> MASMTGGQQMGRGSMPEIVDTCSLASPASVCRTKHLHLRCSVDFTRRTLTGTAALTVQSQEDNLRSLVLDTKDLTIEKVVINGQEVKYALGERQSYKGSPMEISLPIALSKNQEIVIEISFETSPKSSALQWLTPEQTSGKEHPYLFSQCQAIHCRAILPCQDTPSVKLT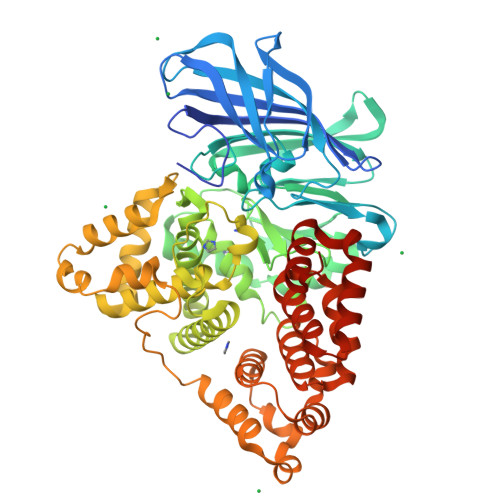YTAEVSVPKELVALMSAIRDGETPDPEDPSRKIYKFIQKVPIPCYLIALVVGALESRQIGPRTLVWSEKEQVEKSAYEFSETESMLKIAEDLGGPYVWGQYDLLVLPPSFPYGGMENPCLTFVTPTLLAGDKSLSNVIAHEISHSWTGNLVTNKTWDHFWLNEGHTVYLERHICGRLFGEKFRHFNALGGWGELQNSVKTFGETHPFTKLVVDLTDIDPDVAYSSVPYEKGFALLFYLEQLLGGPEIFLGFLKAYVEKFSYKSITTDDWKDFLYSYFKDKVDVLNQVDWNAWLYSPGLPPIKPNYDMTLTNACIALSQRWITAKEDDLNSFNATDLKDLSSHQLNEFLAQTLQRAPLPLGHIKRMQEVYNFNAINNSEIRFRWLRLCIQSKWEDAIPLALKMATEQGRMKFTRPLFKDLAAFDKSHDQAVRTYQEHKASMHPVTAMLVGKDLKVDLEHHHHHH>[2x]MAENTEPRIGVFVCHCGTNIAGSMSIDDVVNYAKTLPYVAVADQYQYMCSTPGQKKIDDAIKEYNLTGVVVAACSPRLHEPTFRTATKEGGLNPFRFEMANIREQNSWVHMHGMWDEATQKAKDQVRMAVAKAAKLEDLVPKSVPVEKTAMVVGGGVAGMQAALDLASAGIKTYLIERTPTIGGRMSQLDKTFPTLDCSQCILTPKMVDVGRHPNIEMMTYTEVEKVEGYIGNFDVTLRKKARGVLTPTEATAKGIVGGGCNGCGDCSAVCPVIKPNPFEMGMAPRKAIYIYHAQVMPLIYTVDFDSCVKCGLCVEACGDKKAIDLEMQDEFITVKVGTAVLATGYELFPIENKREWGYKQFDNVINALEFERLICASGPTGGHLVRPSDGKTPMKVGFVLCAGSRDNTGIGKPYCSRFCCMYSLKHAHQIMEKIPGAVAYLFYMDIRSFGKMYEEFYYRIQHEGAKFIRGRVANVLEDKETKNLHVFTEDTLLGRPVDVEVDLLVLAAAVQPNEGANELRKKFGVSASQDGWMLEAHPKLNPCGTTTAGVFLAGVCQGPKDIPDTVAQAEGAASAASIPIHMGEVELEPYFAMCIDELCAGCGMCVNLCPYSALSLGEKNGRTVMVVTEAKCKGCGTCGGFCPGGAIKMQHFTTPQIVAQIDAFFAGGEQ;>[2x]MHEYAFFLGCIAPNRYPGCEASAIKTSEKVGIKLLPLK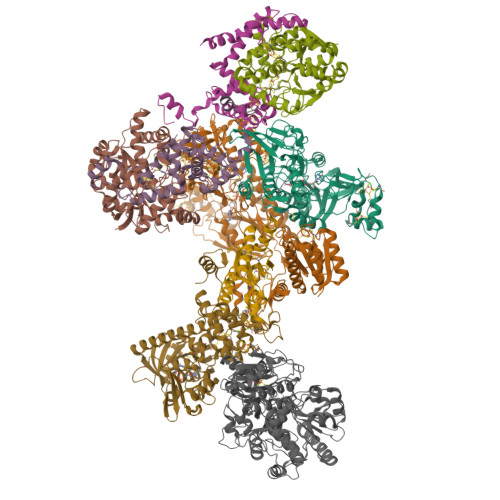GASCCPAPGAFGSIDLNVWYAMAARNLVLAEEMKKDIALICNGCYKSIWEVNHILKHNDELRDNVNEVLAEIDMQFKGTIDVWHLAELYYDDKVCGVQKIKDSVTTPLSGAKVAAHYGCHLMKPKKERHFGDTENPMWFEELIGALGAEPIQYRNKMQCCGAGGGVRGYDIVHALDITNEKLINIQEAGADAITELCPFCQLQFDRGQIEIKEKFGDVYNIPVLHYNELLGLAQGMSPQDLALDLHAIDCTPFLQKVL;>[2x]MAAKSYNIPELDKKLADRRYHLSDTNPEFTQKILKTSRTIANMCYQCGTCTGSCPSAPRSSYRIRLFMRRCVLGLENEALTDPDLWLCTTCYSCTDRCPRDIAPTDVIMAMRNLAFKRDIVPKNFLQTVQLIYNSGHGVPNNDVNRAARTKLGLPADPPTTHSYPEFVKGIQKIIDHYELKENADRILKGD;> MSENSEIMKYVATTCPYCGVGCTLNLVVSNGKVVGVEPNQRSPINEGKLCPKGVTCWEHIHSPDRLTTPLIKKDGKFIEASWDEALDLVAKNLKVIYDKHGPKGLGFQTSCRTVNEDCYIFQKFARVGFKTNNVDNCARICHGPSVAGLSLSFGSGAATNGFEDALNADLILIWGSNAVEAHPLAGRRIAQAKKKGIQIIAVDPRYTMTARLADTYVRFNPSTHIALANSMMYWIIKEGLEDKKFIQDRVNGFEDLKKTVENYADAEAIHGVPLDVVKDIAFRYAKAKNAVIIYCLGITELTTGTDNVRSMGNLALLTGNVGREGVGVNPLRGQNNVQGACDMGAYPNVYSGYQKCEVAENRAKMEKAWSVTNLPDWYGATLTEQINQCGDEIKGMYILGLNPVVTYPSSNHVKAQLEKLDFLVVQDIFFTETCQYADVILPGACFAEKDGTFTSGERRINRVRKAVNPPGQAKEDIHIISELAAKMGFKGFELPTAKDVWDDMRAVTPSMFGATYEKLERPEGICWPCPTEEHPGTPILHREKFATADGKGNLFGIDYRPPAEVADAEYPFTLMTGRLIFHYHSRTQTDRAADLHREVPESYAQINIEDARRLGIKNNEYIKLKSRRGETTTLARVTDEVAPGVVYMTMHFADGVNNLTNTVLDPMSKMPELKHCAISIEKVGGN;> MAAKGDMLYAWAKDAEIQKKGECGGAVTALLKHALETKMVDAVVAIKKGKDLYDAVPTVITNPEDIIQTAGSLHCGTLLIPKLIKKYLNGAKDMKLAVTCKGCDAMAFYELAKRNQINLDNIIMIGVNCGGSVSPVTARKMISNKFGVDPDTVHKEEIDKGQFIIEYEGGHKGIKIDELEEEGYGRRSNCRRCKMKIPRQADIAAGNWGVIGDKAGKATFLEICSEKGANLVNSAQSKGALEISPADPKGIDIRAKVEKAMFNLGDEWRHRDFEGMGKGKDRLKLMMSESSKCIKCYACVEACPICYCIECSTKKPWYIAPGVLPTSFMFHLIRFAHVSDSCINCGQCEELCPMEIPNALFMHSQQVEIEKMFGHIPGQDMTPPIHAFVEEKAERARLDATGTDSIYTNIFTDE;> MADDWKPQILAIICNWCSYAGADLAGGARIQYPPTVRAIRVMCTGRVDMLFILKAFVEGADGVLVSGCHFGDCHYLEGNYKAAKRMFMIKNLLRNIGLDDRRFRMTFVSASEGAKWGMVMEDVTNTIKELGPSPIKEFKK>MESANDKELDQLLNEHFAGRVVRKDLTKLIKEGANVPVYVLEYLLGMYCASDDPEIIEQGLRNVKTVLAENYVRPDEAEKVKSLVRERGSYKVIDRVTVKLNERKDKYEASFSNLGIKDAEISAGIVKEYEKLLVGGIWVIATLSYYFEEGQTSSPFGVSLLKPIQMPNMNMDELFSGRAALSTDQWRESLIRSIGMEPASLKEDVQWHLL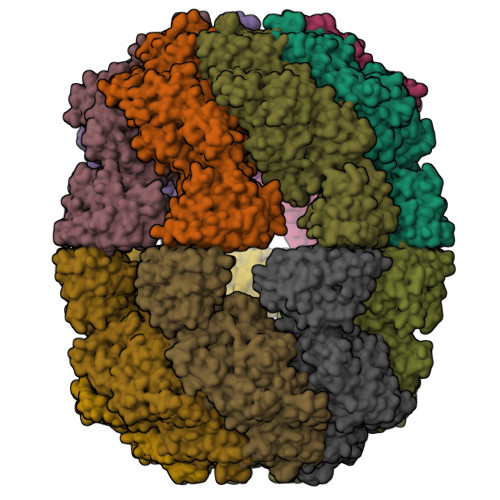ARMVPFVENNYNVCELGPRGTGKSHIYKECSPNSILVSGGQTTVANLFYNMSSRRIGLVGLWDVVAFDEVAGISFKDKDGVQIMKDYMASGSFARGREQMEASASMVFVGNINQSVESLVKTSHLLAPFPEAMIDSAFFDRFHAYIPGWEIPKMRPEFFTNRYGLIVDYLAEFFREMRKRSFADSIEKYFKLGNNLNQRDVIAVRKTVSGLMKLLYPHGQFNKEDVRQCLEYALQVRRRVKEQLKKIGGMEFYDVHFSYIDNDTLEEHFVSVKEQGGGGLIPEGPAKPGFLYTIGLSNKGMPGLYRLELQVTKGSGKLATSGLWNSSSAKEQVKIAFDYFKANASRISGGSKVMEHDFHLHVVELQNTGPLSHLALPSLVAFASGLLGRSVQSQMVVLGDMSLGGSVTPVESIAECLQVAFDAGAKKVALPMSSAADIPTIPVELFTKFQTSFYADPVDAVFKGLGVD[14x]> GSHMRNVAAEQQLRELESTFDGRLGFVALDTATGARIAHRADERFPFCSTFKTMLSAAVLARSAGDAALLQRRIPYAKRDLVRYSPITEKHVGAGMTVAELCAATLQYSDNTAANLLIALLGGPQAVTAYARSIGDATFRLDRRETELNTAIPGDERDTTTPAAMAASVRRLLVGDALGTAQRAQLNAWMLGNKTGDARIRAGVPAGWRVADKTGTGDYGTGNDIGVAYPPDRAPIVFVVYTTMRSRNAQARDDVIASAARIAARAFV

In class A β-lactamases, a conserved structural element called the omega loop5 constitutes a wall at the active site that shapes the binding cavity. PenL (NCBI reference sequence: YP_439646.1) is highly conserved in pathogenic Burkholderia species, including Burkholderia pseudomallei, Burkholderia mallei, and Burkholderia cenocepacia. PenL has been used as a model in exploring various evolutionary paths to substrate spectrum extension through amino acid substitutions, deletions, and duplications. In this study, we demonstrate the extensive perturbation-absorbing capacity of the omega loop against TR mutations of various sizes, some of which are large enough to include the entire omega loop.

Similar to other class A β-lactamases, the active site cavity of PenL-WT can be depicted as a tetrahedral organization, where one plane is open for the substrates, while the other three are composed of the omega loop (residues 161–179), structures including the β3 strand (residues 230–240), and the 102–107 loop and the neighboring 130–132 bend. These three planes meet at the center, where the N-terminal end of the α2 helix, containing the catalytic Ser70, is located. Consistently, the key residues in the active site of PenL-WT were superimposed closely with those in SHV-1, TEM-1, and CTX-M-9. In addition to these common features, PenL-WT showed two unique features in the active site compared to the homologs: an interaction between Arg104 and Thr167 and an increased number of water molecules in the active site. The interaction between Arg104 and Thr167 through a hydrogen bond (2.46 Å) tightened the binding cavity by linking the loop of amino acids 102–107 to the omega loop. Intriguingly, other class A β-lactamases such as SHV-1, TEM-1, and CTX-M-9 do not have such an interaction. The active site of PenL-WT had a fifth water molecule, W5, while class A β-lactamases normally have three to four water molecules, including the catalytic water W1, which has a role in the deacylation reaction of the substrate. All of these water molecules participate in the extensive hydrogen-bond networks that indirectly connect the key active site residues Ser70, Asn132, Glu166, Asn170, and Thr237, which are gathered from all sides of the active site, appropriately positioning them for the catalytic activity. While PenL-WT exhibited catalytic activities (kcat and kcat/Km) with nitrocefin, cefotaxime, penicillin G, and amoxicillin, PenL-tTRs exhibited loss of such activity.> MRGSHHHHHHGSMTQKTIKIGIVGLGRLGKIHATNIATKIQHAKLQAATSVVPAELDWAKKELGVEEVFEDFDDMVQHADIDAVFIVSPSGFHLQQIESALNAGKHVFSEKPIGLDIEAIEHTQQVIAQHANLKFQLGFMRRFDDSYRYAKQLVDQGKIGDITLIRSYSIDPAAGMASFVKFATSANSGGLFLDMSIHDIDVIRWFTGKEIDKVWAIGLNRAYPVLDKAGELETGAALMQLEDKTMAILVAGRNAAHGYHVETEIIGTKGMLRIAQVPEKNLVTVMNEEGIIRPTSQNFPERFAQAFLSEEQAFVNSILNNQDVGITAEDGLQGTKAALALQEAFE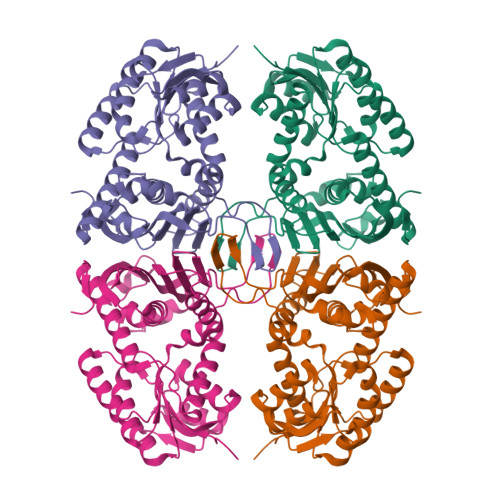KNDIVQVAS>[4x]MRGSHHHHHHGSELPQMTQQLNSDDMQEQLSATRKFSQILSDGNEQIQAVIDAGALPALVQLLSSPNEQILQEALWALSNIASGGNEQIQAVIDAGALPALVQLLS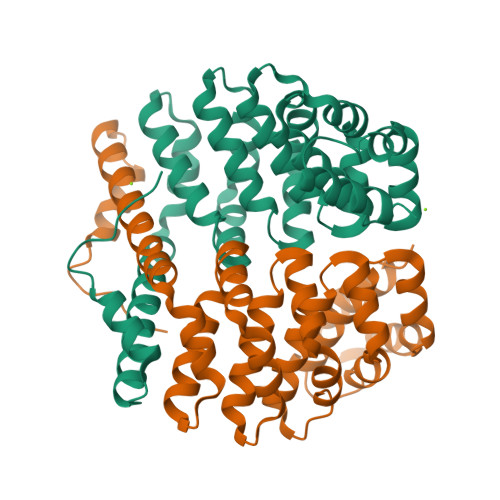SPNEQILQEALWALSNIASGGNEQIQAVIDAGALPALVQLLSSPNEQILQEALWALSNIASGGNEQIQAVIDAGALPALVQLLSSPNEQILQEALWALSNIASGGNEQKQAVKEAGALEKLEQLQSHENEKIQKEAQEALEKLQSH Lactobacillus casei produces a GH29A α-fucosidase, AlfC, that is ~104-fold more active on α(1-6)-fucosyl linkages compared to other linkages. This enzyme is particularly relevant because α(1-6) linkages form the basis of human core fucosylation, which significantly impacts the function of glycoproteins such as antibodies. AlfC is a single-domain enzyme that adopts a (β/α)8 fold typical of GH29 enzymes, with an active site at the center of the barrel. Our results suggest that AlfC employs a conserved hydrolytic mechanism with a specific subsite that accommodates GlcNAc in α(1,6)-linkages, while AlfC tranfucosidase mutants work by shifting equilibrium between open and closed conformations of an active-site loop.

To better understand the catalytic mechanism of AlfCWT and its point mutants, we solved the X-ray crystal structure of AlfCWT into which we soaked l-fucose. In these crystals, fucose produced no substantial conformational changes, with a CαRMSD = 0.14 Å between the fucose-bound and -unbound structures. Fucose binds in an orientation identical to other previously determined fucosidase crystal structures. Specifically, H18, H87, and Y131 coordinate O4 of fucose; E39 and W40 coordinate O3; W40 and H88 coordinate O2; and nucleophile D200 interacts with O1. W283 and W198 contribute to a hydrophobic pocket that accommodates C6. However, there is no structural evidence to support this assignment in any fucosidase, and Oδ of this residue in AlfC is ~9 Å from the nucleophile Oγ, with no plausible access to the reactive C1 of fucose. Its location on an α-helix with very low B-factors suggests it is unlikely to unfold to move closer to C1 of fucose, while its hydrogen bond with O3 makes it far more likely to be involved in fucose binding rather than catalysis. In AlfC, Oδ of this residue is ~12 Å from the nucleophile Oγ, with W198 separating the two residues.

>[4x]MNDNVAWFKQAKYGMMIHWGLYSLLAGEYRGESSSAYAEWIQSKFQIPNAEYGNLATAFNPLYFDAKKIVALAKQCGMQYLVVTTKHHDGFAMYHSKVDAYNVYDATPFHRDIIGELAEACQKAGLKFGLYYSQDLDWHDPNGGGYKSNDVETAGTTWDNSWDFPDEDQKNFDLCFDNKILPQIKEIMSNYGDIATAWFDVPMTLSEAQSQTIYDTVRELQPNCLINSRLGNGKYDFVSLGDNEIPKNKEDMNKTDVDYNEITGFKPSPLGLYETAGTINDSWGFSYHDQNWKTPRTLYRYKQHLNDFGINYLLNVGLDPLGRVPMMAEENLLAAKALEDEANRL In this work, the flexibility of the EF-hand motifs are examined by crystallographic and thermodynamic studies of binding of Pb2+, Ba2+ and Sr2+ to Calcium Binding Protein-1 from Entamoeba histolytica (EhCaBP1). EhCaBP1 has four EF-hand motifs, each of them able to bind one calcium ion similar to that of calmodulin. The overall structure is trimeric in which EF-hand 1 of one molecule interacts with EF-hand 2 of the other molecule in a domain swapped manner to form an assembled domain similar to that of the calmodulin N-terminal domain. Thermodynamic studies confirm that EhCaBP1 has five binding sites for Ba2+ compared to four binding sites for the other metals. These structures and thermodynamic studies reveal that the EF-hand motifs can accommodate several heavy atoms with similar binding affinities.

In CaM, Ba2+ has low binding affinity for EF-hand motifs compared to Ca2+ For EhCaBP1 also, Ba2+ has lower binding energy compared to Ca2+, even though the difference in binding energy is not very high, therefore it cannot replace the calcium at low concentrations. Hence, the EhCaBP1 was denatured and refolded in Ba2+ containing buffer. The overall structure of the Ba2+-EhCaBP1 complex, including the coordination geometry, is similar to that seen in the native structure, except for a couple of features The coordination distances in the EF1 motif are on average 0.1 Å longer in Ba2+-EhCaBP1 than in the Ca2+-bound structure. This difference suggests that the EF-hand motif is flexible enough to accommodate metal ions of varied size. Moreover, a significant difference occurs in the EF2 motif, where two barium sites are observed. One barium is located at the same site as calcium The extra barium is in the close vicinity of EF-hand 2 loop, with partial occupancy and coordinated by residues K43, D46 and D48. Both barium ions in the EF2 motif seem to be partially occupied, according to analyses of temperature factors and difference Fourier peaks. Before placing the heavy atoms, the fully occupied barium ion site had difference Fourier electron density at about 10σ and partially occupied barium ions has about 5σ level, clearly indicating the occupancy level. Our work has also provided the first successful example of replacing Ca2+ with Ba2+ in the EF1 motif of a calcium binding protein.

>[2x]MAEALFKEIDVNGDGAVSYEEVKAFVSKKRAIKNEQLLQLIFKSIDADGNGEIDQNEFAKFYGSIQGQDLSDDKIGLKVLYKLMDVDGDGKLTKEEVTSFFKKHGIEKVAEQVMKADANGDGYITLEEFLEFSL>[2x]GAMGSMATYEVLCEVARKLGTDDREVVLFLLNVFIPQPTLAQLIGALRALKEEGRLTFPLLAECL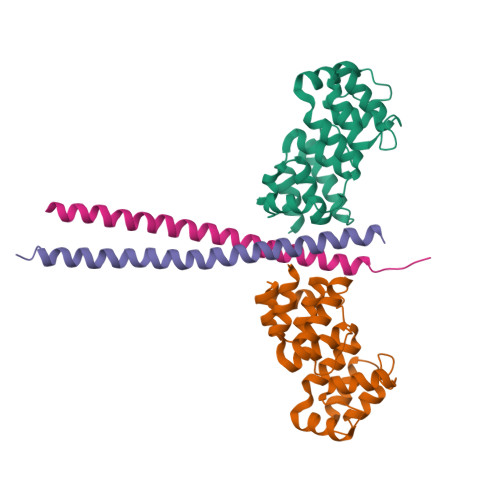FRAGRRDLLRDLLHLDPRFLERHLAGTMSYFSPYQLTVLHVDGELCARDIRSLIFLSKDTIGSRSTPQTFLHWVYCMENLDLLGPTDVDALMSMLRSLSRVDLQRQVQTLMGLHLSGP;>GHMASGSLGELQESQSRLEAATKECQALEGRARAASEQARQLESEREALQQQHSVQVDQLRMQGQSVEAALRMERQAASEEKRKLAQLQVAYHQLFQEYDNHIKSSVVGSERKRGMQLEDLKQQLQQAEE[2x]>[2x]GGNPGDNL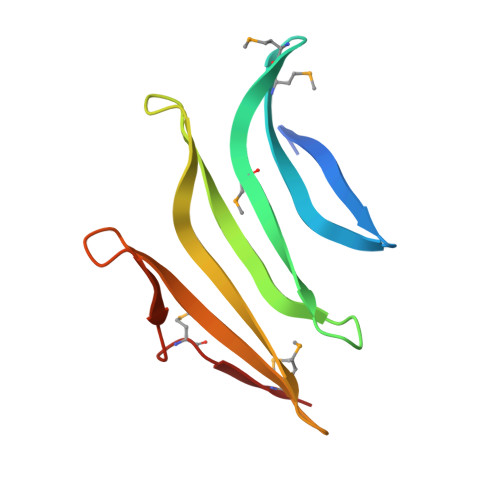IYNAEEVNGVVVSETIFKMEGTMLTNYMKHNYKYDANNQRTEDEAQKWNSNKNRWENNLCIRYTYGNKSMTTEYYKWNSKKKEYILVPEMTVTMDK>SRNNPFYFPSRRFSTRYGNQNGRIRVLQRFDQRSRQFQNLQNHRIVQIEAKPNTLVLPKHADADNILVIQQGQATVTVANGNNRKSFNLDEGHALRIPSGFISYILNRHDNQNLRVAKISMPVNTPGQFEDFFPASSRDQSSYLQGFSRNTLEAAFNAEFNEIRRVLLEENAGGEQEERGQRRWSTRSSENNEGVIVKVSKEHVEELTKHAKSVSKKGSEEEGDITNPINLREGEPDLSNNFGKLFEVKPDKKNPQLQDLDMMLTCVEIKEGALVLPHFNSKAMVIVVVNKGTGNLELVAVRKEQQQRGRREEEEDEDEEEEGSNREVRRYTARLKEGDVFIMPAAHPVAINASSELHLLGFGINAE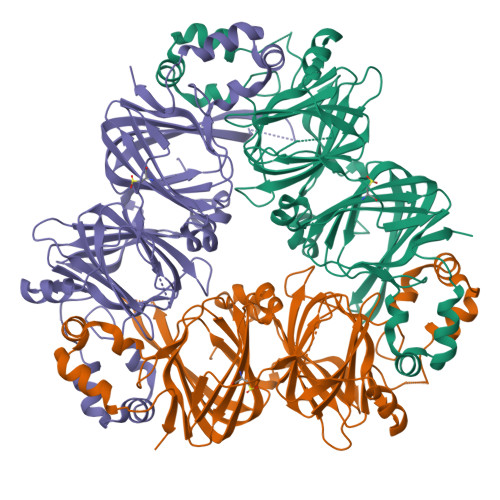NNHRIFLAGDKDNVIDQIEKQAKDLAFPGSGEQVEKLIKNQKESHFVSARP[6x]> GGFKPSRPPRPSRPPPPTPR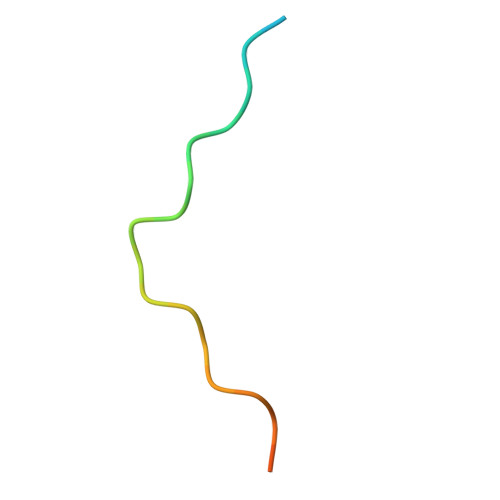RPASV>[2x]GTSMETFDPTELPELLKLYYRRLFPYSQYYRWLNYGGVIKNYFQHREFSFTLKDDIYIRYQSFNNQSDLEKEMQAANPYKIDIGAVYSHRPNQHNTVKLGAFQAQEKELVFDIDMTDYDDVRRCCSSADICPKCWTLMTMAIRIIDRALKEDFGFKHRLWVYSGRRGVHCWVCDESVRKLSSAVRSGIVEYLSLVKGGQDVKKKVHLSEKIHPFIRKSINIIKKYFEEYALVNQDILENKESWDKILALVPETIHDELQQSFQKSHNSLQRWEHLKKVASRYQNNIKNDKYGPWLEWEIMLQYCFPRLDINVSKGINHLLKSPFSVHPKTGRISVPIDLQKVDQFDPFTVPTISFICRELDAISTNEEEKEENEAESDVKHRTRDYKKTSLAPYVKVFEHFLENLDKSRKGELLKKSDLQKDF;>[2x]MEFSGRKWRKLRLAGDQRNASYPHCLQFYLQPPSENISLIEFENLAIDRVKLLKSVENLGVSYVKGTE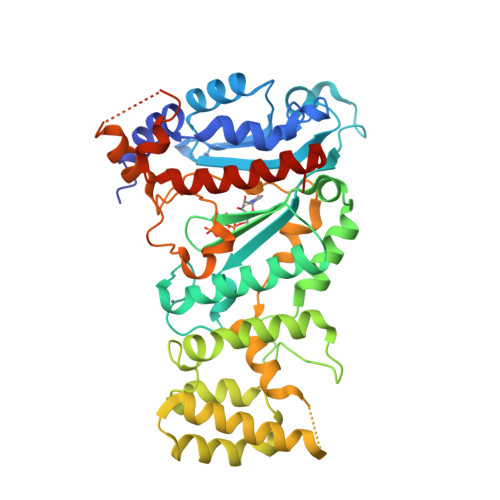QYQSKLESELRKLKFSYRENLEDEYEPRRRDHISHFILRLAYCQSEELRRWFIQQEMDLLRFRFSILPKDKIQDFLKDSQLQFEAISDEEKTLREQEIVASSPSLSGLKLGFESIYKIPFADALDLFRGRKVYLEDGFAYVPLKDIVAIILNEFRAKLSKALALTARSLPAVQSDERLQPLLNHL>MTTATAGLAVELKQSTAQAHEKAEHSTFMSDLLKGRLGVAEFTRLQEQAWLFYTALEQAVDAVRASGFAESLLDPALNRAEVLARDLDKLNGSSEWRSRITASPAVIDYVNRLEEIRDNVDGPALVAHHYVRYLGDL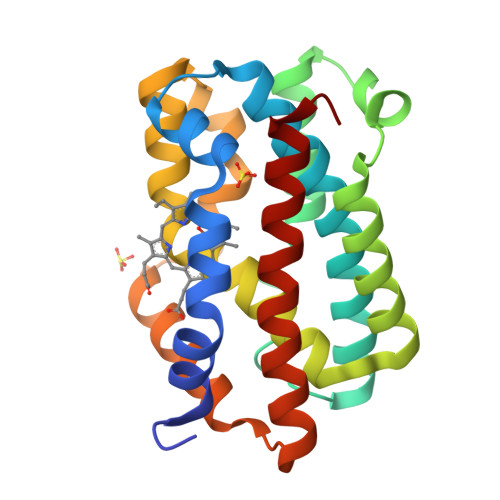SGGQVIARMMQRHYGVDPEALGFYHFEGIAKLKVYKDEYREKLNNLELSDEQREHLLKEATDAFVFNHQVFADLGKGL[3x]>[2x]MSSIKIECVLPENCRCGESPVWEEVSNSLLFVDIPAKKVCRWDSFTKQVQRVTMDAPVSSVALRQSGGYVATIGTKFCALNWKEQSAVVLATVDNDKKNNRFNDGKVDPAGRYFAGTMAEETAPAVLERHQGALYSLFPDHHVKKYFDQVDISNGLDWSLDHKIFYYIDSLSYSVDAFDYDLQTGQISNRRSVYKLEKEEQIPDGMCIDAEGKLWVACYNGGRVIRLDPVTGKRLQTVKLPVDKTTSCCFGGKNYSEMYVTCARDGMDPEGLLRQPEAGGIFKITGLGVKGIAPYSYAG

Senescence marker protein-30 (SMP30) is a 34-kDa protein whose tissue levels in the liver, kidney, and lung decrease with aging. Biochemical studies suggested that SMP30 is a gluconolactonase (GNL, EC 3.1.1.17) and requires a divalent metal ion such as Zn2+ and Mn2+ for its gluconolactonase activity. In the ascorbic acid biosynthesis pathway, the ring structure of d-glucuronate is cleaved to generate l-gulonate, and then a γ-lactone ring, which is a basic structural framework of ascorbic acid, is formed from l-gulonate by SMP30/GNL. The crystal structure showed that human SMP30/GNL adopts a six-bladed β-propeller fold, which is similar to those of squid diisopropyl-fluorophosphatase (DFPase), drug resistance protein 35 (Drp35), and paraoxonase (PON).

The crystal structures of mouse and human SMP30/GNL in the substrate-free form were determined at 1.95 Å and 1.50 Å resolutions, respectively. In the course of the crystallographic refinement, a strong electron density was found inside the β-propeller structure in both mouse and human SMP30/GNL. The ICP-MS analysis suggested that the divalent metal ion bound to SMP30/GNL molecules in the crystal showed heterogeneity; the SMP30/GNL molecules bound Mn2+, Zn2+, Mg2+, or Ca2+ in the crystal. Since Ca2+ was the most abundant metal ion in the purified sample, a Ca2+ ion was placed at the metal site for the crystallographic refinement. The asymmetric unit of the mouse and human SMP30/GNL contained two SMP30/GNL molecules. However, molecular weight analysis with static light scattering revealed that mouse and human SMP30/GNL exist as a monomer in solution. The overall structure of mouse SMP30/GNL was essentially the same as that of human SMP30/GNL. Least-squares fitting of mouse and human SMP30/GNL with corresponding 297 Cα atoms gave a root-mean-square (rms) deviation of approximately 0.6 Å. Since human cells have a loss-of-function genetic mutation on gluconolactone oxidase, which is the last enzyme in the ascorbic acid biosynthesis pathway, human cells cannot synthesize ascorbic acid. Therefore, human SMP30/GNL, the crystal structure of which was determined earlier, may have a biological function other than ascorbic acid biosynthesis.>[2x]SNANYMETGDQRFGDLVFRQLAPNVWQHTSYLDMPGFGAVASNGLIVRDGGRVLVVDTAWTDDQTAQILNWIKQEINLPVA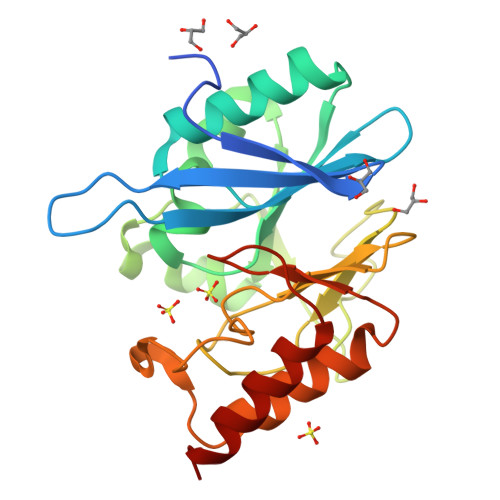LAVVTHAHQDKMGGMDALHAAGIATYANALSNQLAPQEGMVAAQHSLTFAANGWVEPATAPNFGPLKVFYPGPGHTSDNITVGIDGTDIAFGGCLIKDSKAKSLGNLGDADTEHYAASARAFGAAFPKASMIVMSHSAPDSRAAITHTARMADKLR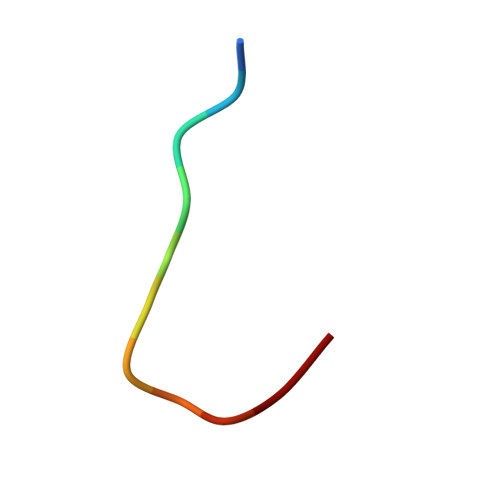> EATVYAGTGRL(2S)-(3-{[AMINO(IMINO)METHYL]AMINO}PHENYL){[(S)-[(1R)-1-({N-[(BENZYLOXY)CARBONYL]-L-TYROSYL}AMINO)-2-METHYLPROPYL](HYDROXY)PHOSPHORYL]OXY}ACETIC ACID | C30 H36 N5 O9 P | 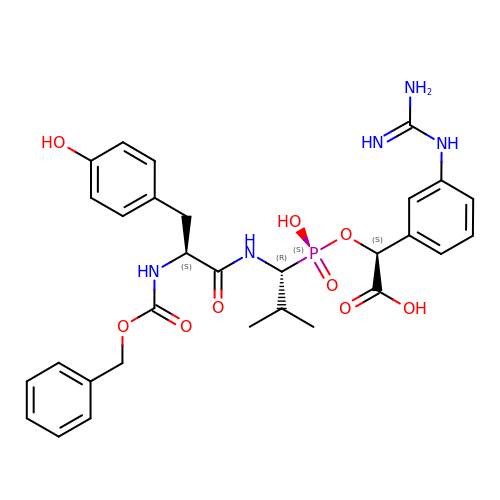YRZNVYCMTZKRPJ-OHSXHVKISA-N N-carboxyl-N-methyl-beta-muramic acid | C11 H19 N O9 | 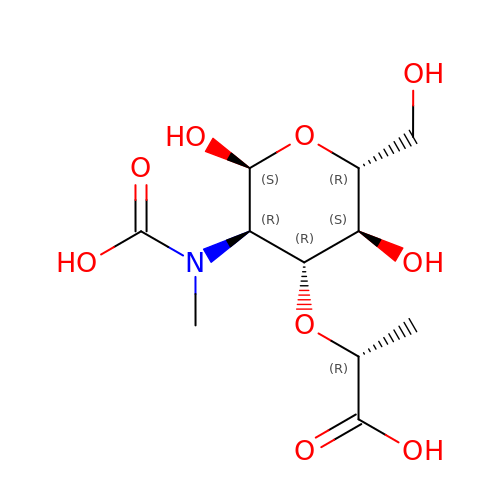PVOFHMJNZUCTDT-MXGCPANSSA-N>[2x]MHHHHHHMKLTIERAALLKALGHVQSVVERRNTIPILSNILLSAEGDRLSFSATDLDMEIIDEGFAQIDVPGQITAPAH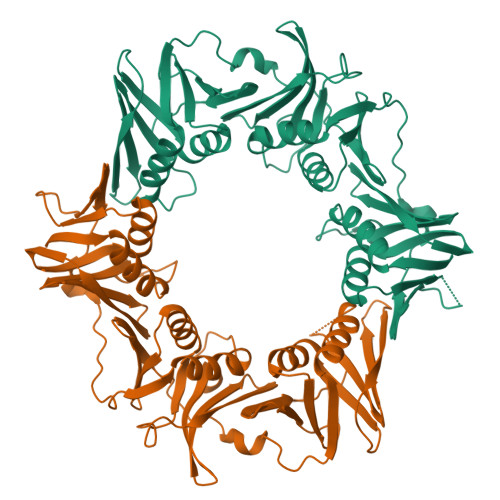TLYEIVRKLPDGADVSLSFSGDDPRLVIQAGRSRFNLPVLPAGDFPVMSSDGLSSRIAVDTNELIRLIDKTRFAISTEETRYYLNGLYVHTVNEGGETKLRAVATDGHRLALAEMPAPEGAVGIPGVIVPRKTIAEARRLMESAGETVDLQVSPQKVRFEFGAAALTSKVIDGAFPDYMRVIPRDNAKILTLDNDLFAKAVDRVATISAEKSRSVKLAVEPGRITLTVRNMEAGQAVEEVEVDYDGEPFEIGFNARYLLDVCGQIAGPQAEFRFADPASPTLVVDPVDPGVKYVLMPLRV> MAKKTPPVVFHWFPFIGSTISYGIDPYKFFFDCRAKYGDIFTFILLGKKTTVYLGTKGNDFILNGKLRDVCAEEVYSPLTTPVFGRHVVYDCPNAKLMEQKKFVKYGLTSDALRSYVPLITDEVESFVKNSPAFQGHKGVFDVCKTIAEITIYTASRSLQGKEVRSKFDSTFAELYHNLDMGFAPINFM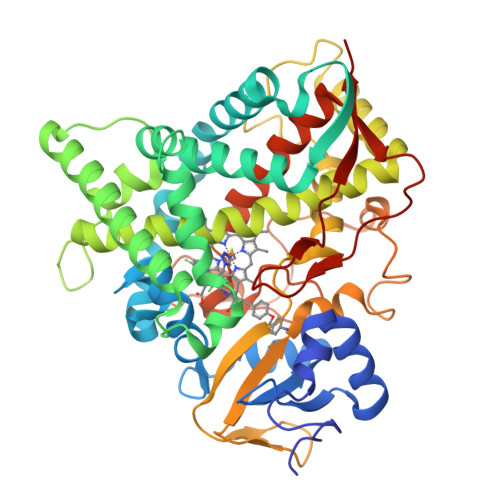LPWAPLPHNRKRDAAQRKLTETYMEIIKARRQAGSKKDSEDMVWNLMSCVYKNGTPVPDEEIAHMMIALLMAGQHSSSSTASWIVLRLATRPDIMEELYQEQIRVLGSDLPPLTYDNLQKLDLHAKVIKETLRLHAPIHSIIRAVKNPMAVDGTSYVIPTSHNVLSSPGVTARSEEHFPNPLEWNPHRWDENIAASAEDDEKVDYGYGLVSKGTNSPYLPFGAGRHRCIGEQFAYLQLGTITAVLVRLFRFRNLPGVDGIPDTDYSSLFSKPLGRSFVEFEKRH> GGACCUCGCAAGGGUAUCAUGGCGGACGACCGGGGUUCGAACCCCGGAUCCGGCCGUCCGCCGUGAUCCAUGCGGUUACCGCCCGCGUGUCGAACCCAGGUGUGCGAGGUCC

The multifunctional VA RNAs interfere with essentially all host systems that interface with double-stranded RNAs (dsRNAs), from their sensing by protein kinase R (PKR), export by Exportin-5, processing by Dicer, editing by ADAR, to activation of oligoadenylate synthetases (OAS), etc. PKR is a central component of the interferon response and the best-characterized target of VA RNAs. To counter the debilitating restriction by PKR, nearly all known viruses have evolved protein or RNA antagonists to evade or inactivate PKR. Among the expanding collection of PKR-regulatory RNAs, VA-I is the best-characterized RNA antagonist.

To address these open questions and understand how viral RNAs employ unique tertiary structures to confound and defeat host immune proteins, we determined a 2.7 Å crystal structure of the apical and central domains of VA-I RNA of adenovirus serotype 2. This RNA is derived from the Dicer-processed form and contains all the elements necessary for PKR inhibition (ΔTS for deletion of terminal stem). The VA-I structure assumes a sharply bent “V” shape, in which two arms of coaxially stacked helices converge at a stable central domain. The SAXS envelopes of VA-I generally showed obtuse angles between the apical and terminal stems, while the crystal structure captures VA-I in an acutely bent “V” shape (~60° between the two arms). In contrast to a proposed 8-nt flexible loop, the apical region of VA-I is highly structured and heavily stacked, explaining its extraordinary thermostability, aberrant gel mobility, and resistance to denaturation by 6 M urea. A stack of two G–C pairs and a G·U wobble pair form the apical core, against which rests a string of three single-stranded cytosines (C67–C69) that form a continuous stack. The apical stem forms an underwound, imperfect A-form duplex of 22 base pairs (bp) that contains four interspersed wobble pairs (three G·U and one A+·C). Instead, they base pair to juxtapose the apical stem with the tetrastem to form an extended coaxial stack spanning 30 layers, just below the threshold of significant PKR activation (~33–35 bp). Unexpectedly, our structure revealed a base triple between the tetrastem (the G39–C120 pair) and C93. The proximal end of the tetrastem is affixed to the central domain through reciprocal nucleobase-2'-OH hydrogen bonds between A123 and G106, each capping a helix through cross-stand stacking.>[7x]XXXXXXXXXXXXXXXXXXXXXXXXXXXXXXXXXXXXXXXXXXXXXXXXXXXXXXXXXXXXXXXXXXXXMIAELFTNNALNLVIIFGSCAALILMSFWFRRGNRKRKGFLFHAVQFLIYTIIISAVGSIINYV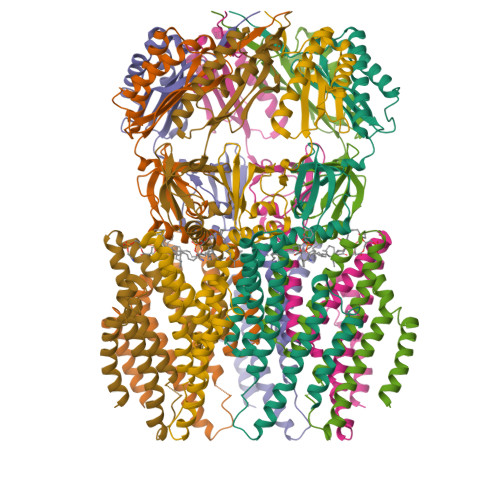IENYKLKFITPGVIDFICTSLIAVILTIKLFLLINQFEKQQIKKGRDITSARIMSRIIKITIIVVLVLLYGEHFGMSLSGLLTFGGIGGLAVGMAGKDILSNFFSGIMLYFDRPFSIGDWIRSPDRNIEGTVAEIGWRITKITTFDNRPLYVPNSLFSSISVENPGRMTNRRITTTIGLRYEDAAKVGVIVEAVREMLKNHPAIDQRQTLLVYFNQFADSSLNIMVYCFTKTTVWAEWLAAQQDVYLKIIDIVQSHGADFAFPSQTLYMDNITPPEQGRLEHHHHHH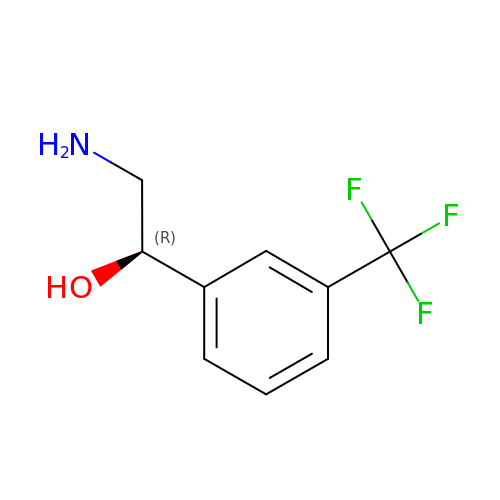(1R)-2-amino-1-[3-(trifluoromethyl)phenyl]ethanol | C9 H10 F3 N O | RRBRWAPWPGAJMA-QMMMGPOBSA-N> GASAGSSKRLRKKDDGKCPLNPHSHLGTYGV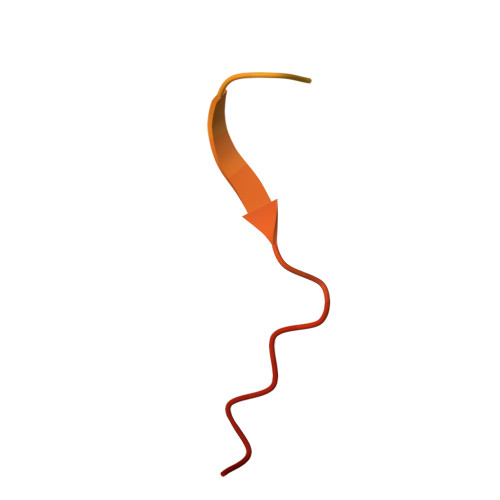FTNAAYDPTP> SNAMPVNKLELLPAVDVRDGQAVRLVHGVSGSETSYGSPLEAALAWQASGAEWLHLVDLDAAFGTGDNRALVAEITGAMDIKVELSGGIRDDASLAAALATGCTRVNLGTAALETPEWAAKAIAEHGDRIAVGLDVRGTTLKGRGWTSEGGDLYETLARLDSEGCARYVVTDIGKDGTLTGPNLELLKNVCAATDRPVVASGGISS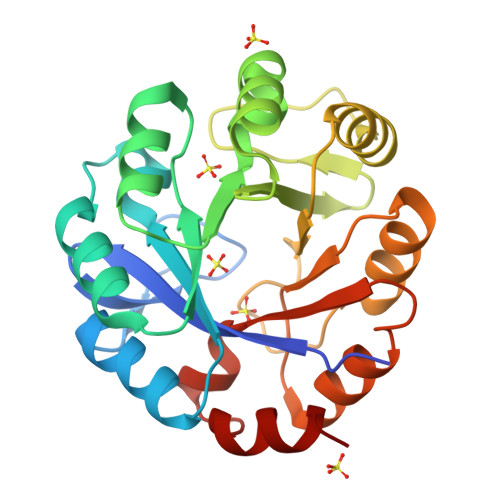LEDLRALAALVPQGVEGAIVGKALYAKAFTLEEALKVVSA> SSS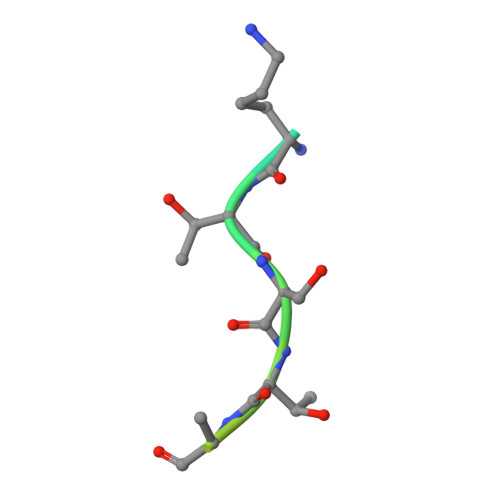ASKTSTNATSSSCATPS FARP1 (FERM, RhoGEF and pleckstrin domain-containing protein 1) and its close homolog FARP2 were identified as guanine nucleotide exchange factors (GEFs) for RhoGTPases that play regulatory roles in neuronal development. FARP1 and FARP2 share a conserved domain architecture, containing a N-terminal 4.1, ezrin, radixin and moesin (FERM) domain, which is followed by a long linker (~200 residues) that connects to a Dbl-homology (DH) domain and two pleckstrin homology (PH) domains. We determined crystal structures of the FERM domains of zebrafish FARP1 (zfFARP1), mouse FARP2 (mFARP2) and zebrafish FARP2 (zfFARP2). As expected from their high degree of sequence identity (>60%), the structures of these FERM domains are very similar to one another, with root mean square deviations within 1.0 Å.

The FERM domain in FARP1 mediates interactions with the intracellular sequences of the transmembrane proteins PlexinA4 and SynCAM 15,8. While the FERM domains in FARP1 and DAL-1 only share ~40% sequence identity, the residues in the binding groove of these two FERM domains are nearly identical as shown by the structural superimposition, strongly suggesting that the interaction between FARP1 and SynCAM 1 uses the same binding mode. We mutated Trp306 in human FARP1 to glutamate (W306E) to disrupt FARP1-SynCAM 1 interactions. According to the FERM/SynCAM 1 binding mode discussed above, Trp306 (corresponding to Trp308 in zebrafish FARP1) is important for interacting with the “GXY” motif in SynCAM 1. The corresponding site in the FERM domains of FARP1 and FARP2 contains a negatively charged residue (Asp97, Glu100 and Asp107 in zfFARP1, mFARP2 and zfFARP2, respectively), suggesting that it cannot serve as a phosphatidylinositol binding site in these FERM domains. Overall, the surface of these FERM domains show highly polarized surface electrostatic potential, with one side positively charged while the opposite side negatively charged. According to the binding mode between the FARP1 FERM and SynCAM 1 proposed above, the side of the FERM domain proximal to the membrane displays positive electrostatic potential. The positively charged surface on the FERM domain likely interacts with the negatively charged lipid membrane surface, thereby facilitating the membrane localization of FARP1 and its interaction with SynCAM 1. In particular, the FERM domains of FARP1 and FARP2 contain a Lys-Arg-Lys-Arg (KRKR) motif in the loop connecting strands β5 to β6 in the F3 subdomain, which is highly conserved in FARP1/2 from different species. A similar motif is also present in FRMD7 (FERM domain-containing protein 7), which has a FERM domain that is closely related to that in FARP1 and FARP2 (~60% sequence identity). The KRKR motif constitutes a major part of the positively charged surface, and may serve as a lipid binding site for targeting FARP1/2 to the plasma membrane.

> SGRQISIRVQMLDDTQEVFEVSQRAPGKALFDLVCSHLNLVEGDYFGLEFQDQRKMIVWLDLLKPILKQIRRPKNIILRFVVKFFPPDHTQLLEELTRYLFALQIKHDLACGRLTCNESSAALLVAHIVQSEIGDFDEVQCKQHLLNNKYIPEQDTLMDKIIGYHRKHVGQTPAESDYQLLEIARRLEMYGVRLHPAKDREGTRLSLAVAHSGVLVFQGHTKINAFNWSKVRKLSFKRKRFLIKLRPDLNSNCQDTLEFMMGSRDCCKVFWKICVEYHAFFRLFE>MTMITPSLHQFPGLANKTYFNFGGQGILPTVALEAITAMYGYLQENGPFSIAANQHIQQLIAQLRQALAETFNVDPNTITITDNVTTGCDIVLWGLDWHQGDEILLTDCEHPGIIAIVQAIAARFGITYRFFPVAATLNQGDAAAVLANHLGPKTRLVILSHLLWNTGQVLPLAEIMAVCRRHQGNYPVRVLVDGAQSAGSLPLDFSRLEVDYYAFTGHKWFAGPAGVGGLYIHGDCLGEINPTYVGWRSITYGAKGEPTGWAEGGKRFEVATSAYPQYAGLLAALQL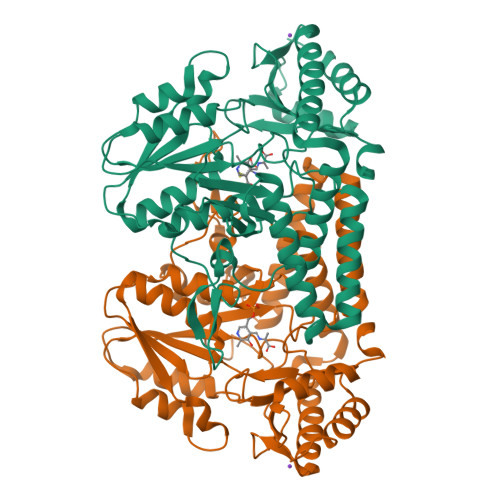HQRQGTAEERYQAICQRSEFLWRGLNQLPHVHCLATSAPQAGLVSFTVDSPLGHRAIVQKLEEQRIYLRTIADPDCIRACCHYITDEEEINHLLARLADFGP[2x]> MGHHHHHHAENLYFQGADPFESYNPEFFLYDIFLKFCLKYIDGEICHDLFLLLGKYNILPYDTSNDSIYACTNIKHLDFINPFGVAAGFDKNGVCIDSILKLGFSFIEIGTITPRGQTGNAKPRIFRDVESRSIINSCGFNNMGCDKVTENLILFRKRQEEDKLLSKHIVGVSIG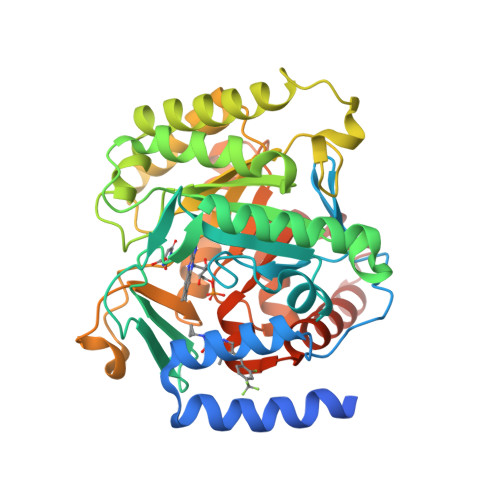KNKDTVNIVDDLKYCINKIGRYADYIAINVSSPNTPGLRDNQEAGKLKNIILSVKEEIDNLEKNNIMNDEFLWFNTTKKKPLVFVKLAPDLNQEQKKEIADVLLETNIDGMIISNTTTQINDIKSFENKKGGVSGAKLKDISTKFICEMYNYTNKQIPIIASGGIFSGLDALEKIEAGASVCQLYSCLVFNGMKSAVQIKRELNHLLYQRGYYNLKEAIGRKHSKS5-amino-2-((6-methoxy-2-methyl-1,2,3,4-tetrahydroisoquinolin-7-yl)amino)-8-(2-(trifluoromethyl)benzyl)pyrido[2,3-d]pyrimidin-7(8H)-one 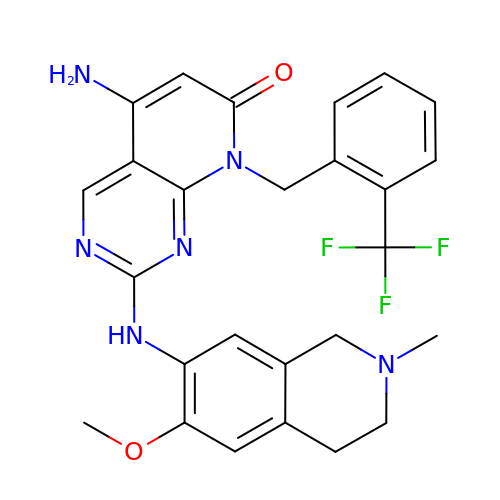| C26 H25 F3 N6 O2 | LQUUWQNDKXYUCK-UHFFFAOYSA-N>AFYNITLRTNDGEKKIECNEDEYILDASERQNVELPYSCRGGSCST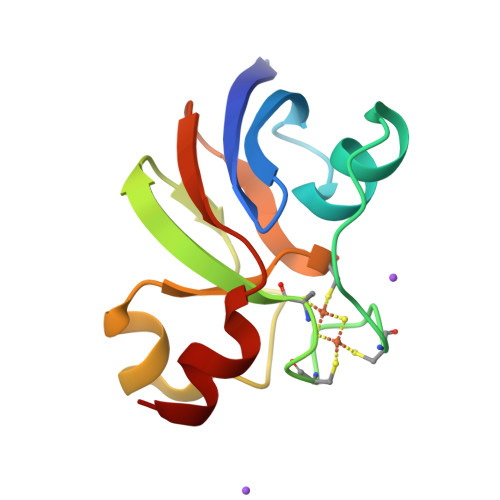CAAKLVEGEVDNDDQSYLDEEQIKKKYILLCTCYPKSDCVIETHKEDELHDM[2x]>[12x]AALSLEPEALQIADNEGTEAALSWLQARPGIQSDRSNWLLRLLMARVAEQTGKNDLALHLLAELDERATRLTLSQWEPELVFEVKARRLKLLRMKSAK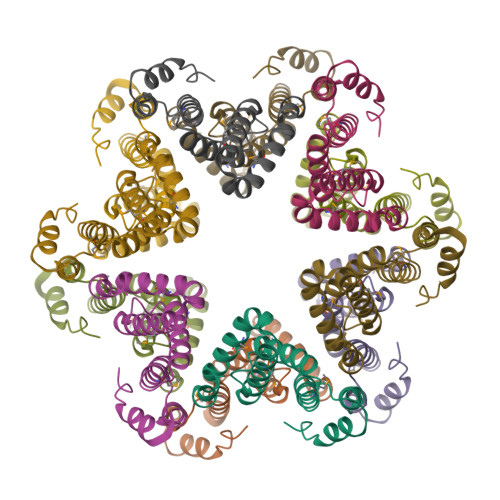TESDRVRLQPDMEHLLAGLIAIDAARAAVLCNS> HHHHHHSENLYFQGMGTPPGLQTDCEALLSRF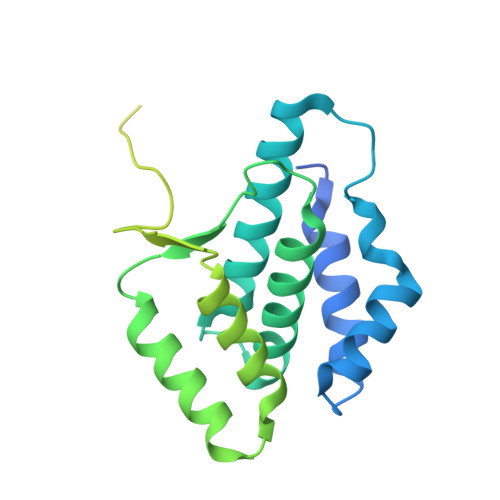QETDSVRFEDFTELWRNMKFGTIFCGRMRNLEKNMFTKEALALAWRYFLPPYTFQIRVGALYLLYGLYNTQLCQPKQKIRVALKDWDEVLKFQQDLVNAQHFDAAYIFRKLRLDRAFHFTAMPKLLSYRMKKKIHRAEVTEEFKDPSDRVMKLITSDVLEEMLNVHDHYQNMKHVISVDKSKPDKALSLIKDDFFDNIKNIVLEHQQWHKDRKNPSLKSKTNDGEEKMEGNSQETERCERAESLAKIKSK We set out to design sets of interacting protein pairs for constructing reconfigurable assemblies. We instead sought to use implicit negative design by introducing three properties that collectively make self associated states unlikely to have low free energy: First, in contrast to the flexible coiled coils and helical hairpins in previous designs, we aimed for well folded individual protomers stabilized by substantial hydrophobic cores; this property limits the formation of slowly-exchanging homo-oligomers. Second, we constructed interfaces in which each protomer has a mixed alpha-beta topology and contributes one exposed beta strand to the interface, giving rise to a continuous beta sheet across the heterodimer interface. Our implicit negative design principles enable the de novo design of heterodimer pairs for which the individual protomers are stable in solution and readily form their target heterodimeric complexes upon mixing, unlike previously designed assemblies.

We determined the crystal structures of two class one designs, LHD29 (2.2 Å) and LHD29A53/B53 (2.6 Å) in which both protomers are fused to DHR53. In the central extended beta sheet, the LHD29 design closely matches the crystal structure (red and green box and Table S5). Aside from backbone beta sheet hydrogens bonds, this part of the interface is supported by primarily hydrophobic packing interactions between the side chains of each interface beta edge strand. The two flanking helices on opposite sides of the central beta sheet (blue and orange box) contribute predominantly polar contacts to the interface, and are also similar in the crystal structure and design model. Apart from crystal contact induced subtle backbone rearrangements in strand 2 of LHD29B that promote the formation of a polar interaction network (blue box), most interface sidechain-sidechain interactions agree with the design model. Association rates were quite fast and ranged from 106 M−1 s−1 for the fastest heterodimer to 102 M−1 s−1 for the slowest heterodimer LHD29, which is still an order of magnitude faster than the fastest associating designed helical hairpin heterodimer DHD37 (10). LHD275A, LHD278A, LHD317A, and a redesigned version of LHD29 with a more polar interface (LHD274) were also predominantly monomeric. For the C4-symmetric hub in the absence of its binding partner we observed an additional concentration-dependent peak on SEC, indicating formation of a higher-order complex. This is likely a dimer of C4 hubs, since the C4 hub contains the redesigned protomer LHD274B, that despite its reduced homodimerization propensity compared to parent design LHD29B still weakly homodimerizes.

>SGGSTWQWVLINISEEARQRIEEYVRRISKKEGTEVHFEKDDGVLHIRVKNLHEKRAREIHEYAKRVIL[2x];>[2x]SGGSSSIFLLSNVSEEARQRAEEYVRRISKKEGTEVRFEKDDGFLTIEVKNLSEERLREIAEYLWRVAV>HHHHHHSSGLVPRGSHMTDIRSETAELRAELVERVHKFGPVFADGVAEGERERRLPDATVRAIDQSQLAMLWTAKSYGGLETDVRTMSEVAKVLSHYCPSTSWVVNNVNGSNLLASKFPRAALDEVFGDAPGAKLASVFAAAGTAVRTPGGYRLTGSWPYGTGILHDDWAILVAREVDADGEPVGGLSMLVPARDLTVEDTWHTVGMRATGSHTVVLRDTFVPEHRVISGELQRSRESATDLGLPPLFRTAAIAAMAVVCASVVLGAGQAARALVVEKAPTRGIAPSKYTRQTDSRTFVSSLGRT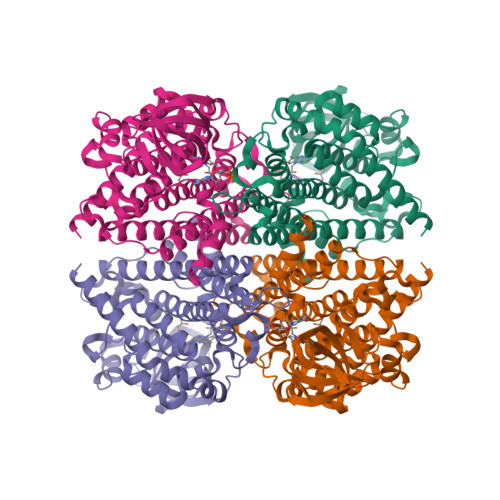ALSIDAAEMHVARAATALDDAAYDAVALPDSELLRIRGDVGQAVSLVTTALDELLWAHGAASFAESNPLQRYWRDANTAARHAMLNVHVGHELYGGSFFGLDPIVPSL[24x]>MVAVEQSEASRLGPVFDSCRANNRAALIGYLPTGYPDVPASVAAMTALVESGCDIIEVGVPYSDPGMDGPTIARATEAALRGGVRVRDTLAAVEAISIAGGRAVVMTYWNPVLRYGVDAFARDLAAAGGLGLITPDLIPDEAQQWLAASEEHRLDRIFLVAPSSTPERLAATVEASRGFVYAASTMGVTGARDAVSQAAPELVGRVKAVSDIPVGVGLGVRSRAQAAQIAQYADGVIVGSALVTALTEGLPRLRALTGELAAGVRLGMSAHHHHHH[4x];>[4x]MSAAIAEPTSHDPDSGGHFGGPSGWGGRYVPEALMAVIEEVTAAYQKERVSQDFLDDLDRLQANYAGRPSPLYEATRLSQHAGSARIFLKREDLNHTGSHKINNVLGQALLARRMGKTRVIAETGAGQHGVATATACALLGLDCVIYMGGIDTARQALNVARMRLLGAEVVAVQTGSKTLKDAINEAFRDWVANADNTYYCFGTAAGPHPFPTMVRDFQRIIGMEARVQIQGQAGRLPDAVVACVGGGSNAIGIFHAFLDDPGVRLVGFEAAGDGVETGRHAATFTAGSPGAFHGSFSYLLQDEDGQTIESHSISAGLDYPGVGPEHAWLKEAGRVDYRPITDSEAMDAFGLLCRMEGIIPAIESAHAVA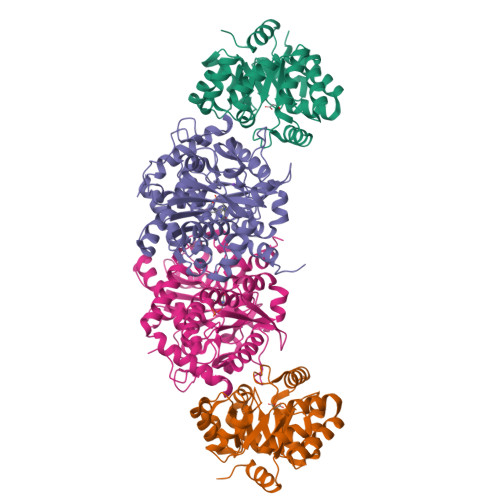GALKLGVELGRGAVIVVNLSGRGDKDVETAAKWFGLLGND>[2x]GASEGEKHITVT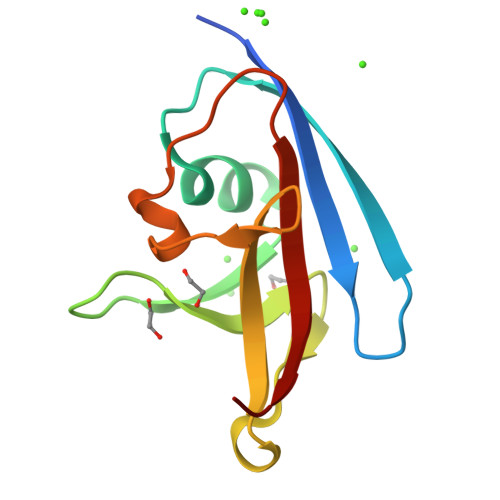VIHGDQTENVFEFDTDAKYLGEVLESENLVDGESGEYGLFITTVDEETADDSKQQWWCITKGGEQVNTSADQTPVSDGDAFELTLKEGY>[4x]RPNHTIYINNLNEKIKKDEL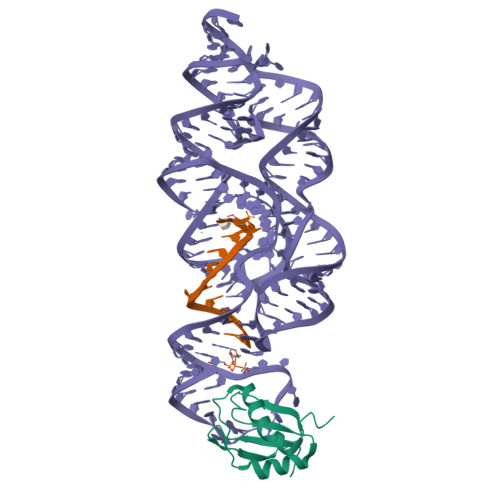KKSLHAIFSRFGQILDILVSRSLKMRGQAFVIFKEVSSATNALRSMQGFPFYDKPMRIQYAKTDSDIIAK>[4x]MRISIFGLGYVGAVCAGCLSARGHEVIGVDVSSTKIDLINQGKSPIVEPGLEALLQQGRQTGRLSGTTDFKKAVLDSDVSFICVGTPSKKNGDLDLGYIETVCREIGFA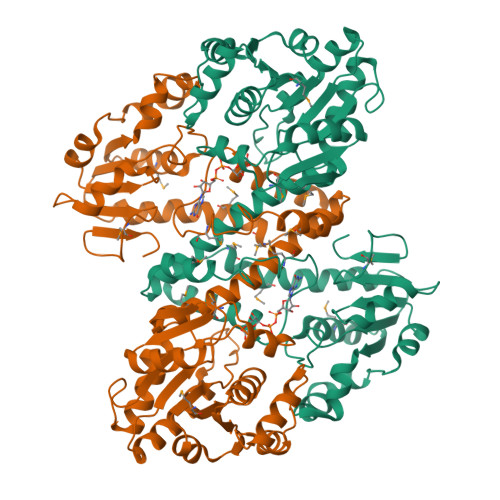IREKSERHTVVVRSTVLPGTVNNVVIPLIEDCSGKKAGVDFGVGTNPEFLRESTAIKDYDFPPMTVIGELDKQTGDLLEEIYRELDAPIIRKTVEVAEMIKYTCNVWHAAKVTFANEIGNIAKAVGVDGREVMDVICQDHKLNLSRYYMRPGFAFGGSCLPKDVRALTYRASQLDVEHPMLGSLMRSNSNQVQKAFDLITSHDTRKVGLLGLSFKAGTDDLRESPLVELAEMLIGKGYELRIFDRNVEYARVHGANKEYIESKIPHVSSLLVSDLDEVVASSDVLVLGNGDELFVDLVNKTPSGKKLVDLVGFMPHTTTAQAEGICW>MASGNARIGKPAPDFKATAVVDGAFKEVKLSDYKGKYVVLFFYPLDFTFVCPTEIIAFSNRAEDFRKLGCEVLGVSVDSQFTHLAWINTPRKEGGLGPLNIPLLADVTRRLSEDYGVLKTDEGIAYRGLFIIDGKGVLRQITVNDLPVGRSVDEALRLVQAFQYTDEHG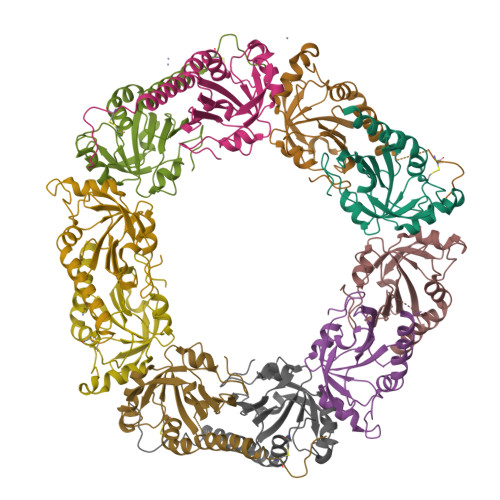EVCPAGWKPGSDTIKPNVDDSKEYFSKHN[10x]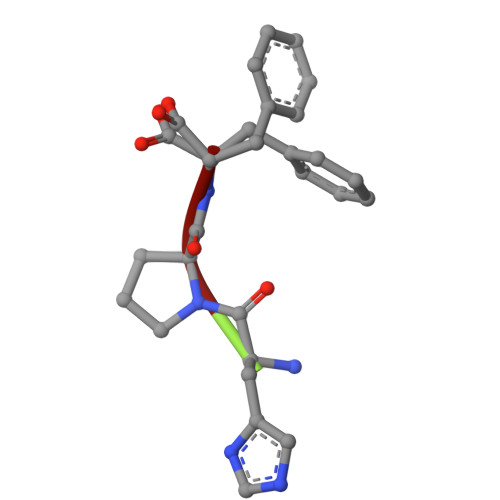> HPF>[2x]KELLDSDGDILRNGGTYYI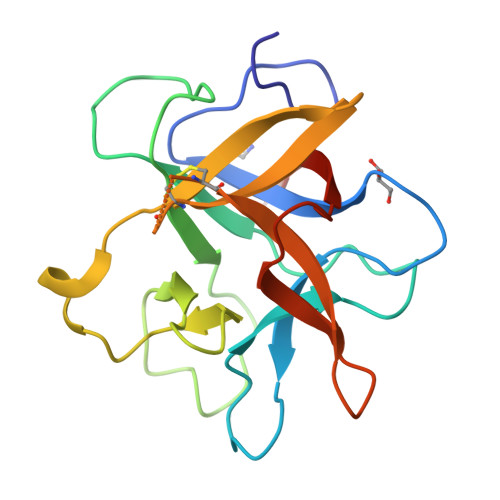LPALRGKGGGLELAKTGDETCPLNVVQARSETKRGRPAIIWTPPRIAILTPAFYLNIEFQTRDLPACLEEYSRLPWKVEGESQEVKIAPKEEEQHLFGSFKIKPYRDDYKLVYCEGNSDDDSCKDLGISIDDENNRLLVVKDGDPLAVRFVKAHRRG> MMSMLVVVTENVPPRLRGRLAIWLLEVRAGV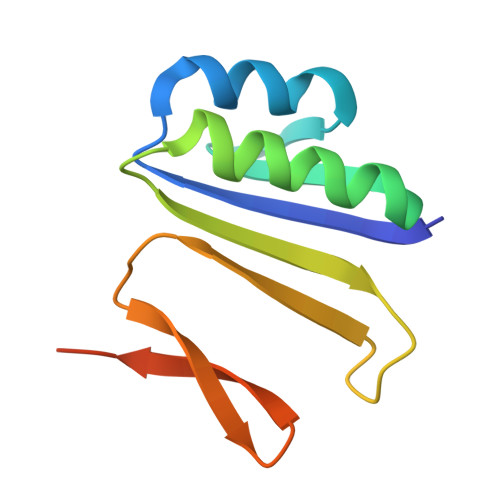YVGDVSAKIREMIWEQIAGLAEEGNVVMAWATNTETGFEFQTFGLNRRTPVDLDGLRLVSFLPVGSSENLYFQ>GSHMSYNNIPAGKDAPNDIYVIIEIPANAAPIRYEIDKDSDALFVDRFMGTAMFYPANYGYVPNTLSEDGDPLDVLVVTPYP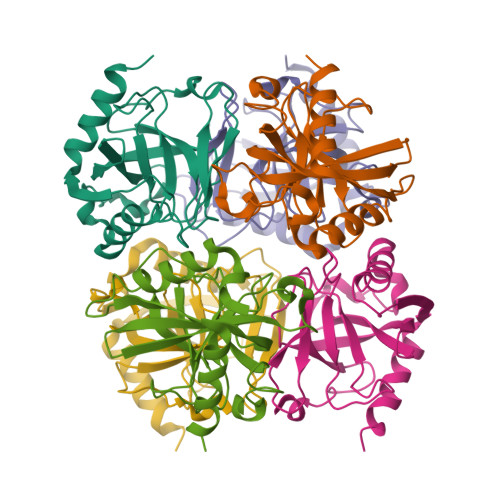VAAGSVIRCRPVGKLNMEDDGGIDAKLIAVPHEKLSPLYKDVKEYTDLPQLLINQVEHFFSHYKDLEPGKWVKISGWEGADVAKAEVIKAIEAAK[8x]> S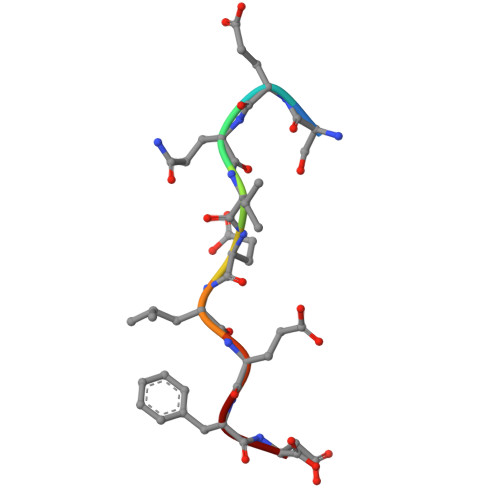EQVELEFD>MSFTVIIPARFASSRLPGKPLADIKGKPMIQHVFEKALQSGASRVIIATDNENVADVAKSFGAEVCMTSVNHNSGTERLAEVVEKLAIPDNEIIVNIQGDEPLIPPVIVRQVADNLAKFNVNMASLAVKIHDAEELFNPNAVKVLTDKDGYVLYFSRSVIPYDRDQFMNLQDVQKVQLSDAYLRHIGIYAYR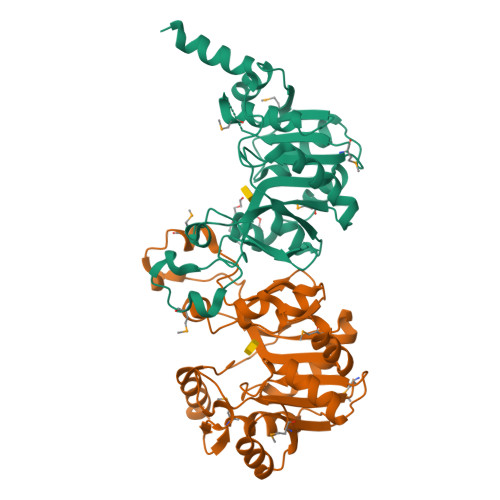AGFIKQYVQWAPTQLENLEKLEQLRVLYNGERIHVELAKEVPAVGVDTAEDLEKVRAILAANLEHHHHHH[2x]>GPLGSSKTKPFTLPILTISEMSNSRFPVPIDSLHTSPTENIVVQCQNGRVTLDGELMGTTQLLPSQICAFRGTLTRSTSRASDQADTPTPRLFNYYWHIQLDNLNGTPYDPAEDIPAPLGTPDFRGKVFGVASQRNPDSTTRAHEAKVDTTSGRFTPKLGSLEITTESDDFDPNQPTKFTPVGVGVDNEAEFQQWSLPNYSGQFTHNMNLAPAVAPNFPGEQLLFFRSQLPSSGGRSNGVLDCLVPQEWVQHFYQESAPAQTQVALVRYVNPDTGRVLFEAKLHKLGFMTIAKNGDSPITVPPNGYFRFESWVNPFYTLAPM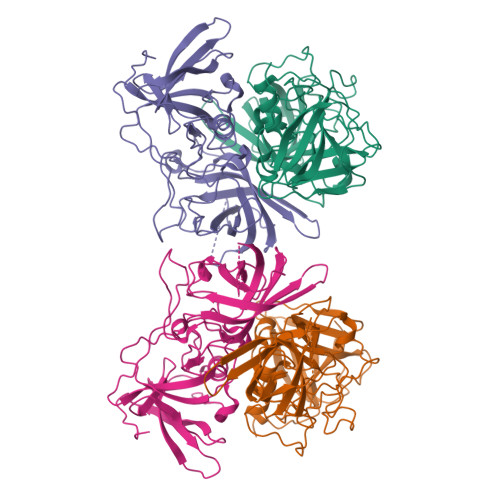GTGNG[4x]> GSGEPREEAGALGPAWDESQLRSYSFPTRPIPRLSQSDPRAEELIENEEPVVLTDTNLVYPALKWDLEYLQENIGNGDFSVYSASTHKFLYYDEKKMANFQNFKPRSNREEMKFHEFVEKLQDIQQRGGEERLYLQQTLNDTVGRKIVM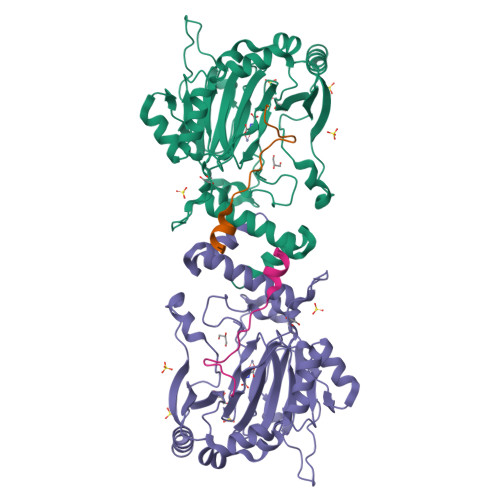DFLGFNWNWINKQQGKRGWGQLTSNLLLIGMEGNVTPAHYDEQQNFFAQIKGYKRCILFPPDQFECLYPYPVHHPCDRQSQVDFDNPDYERFPNFQNVVGYETVVGPGDVLYIPMYWWHHIESLLNGGITITVNFWYKGAPTPKRIEYPLKAHQKVAIMRNIEKMLGEALGNPQEVGPLLNTMIKGRYN;> DIAALLIAAGADVNAHAKGAFF> GLPTMNTPGSCQFLTSDDFQSPSAMPQYDVTPEMRIPGEVKNLMEIAEVDSVVPVQNVGEKVNSMEAYQIPVRSNEGSGTQVFGFPLQPGYSSVFSRTLLGEILNYYTHWSGSIKLTFMFCGSAMATGKFLLAYSPPGAGAPTKRVDAMLGTHVIWDVGLQSSCVLCIPWISQTHYRFVASDEYTAGGFITCWYQTNIVVPAD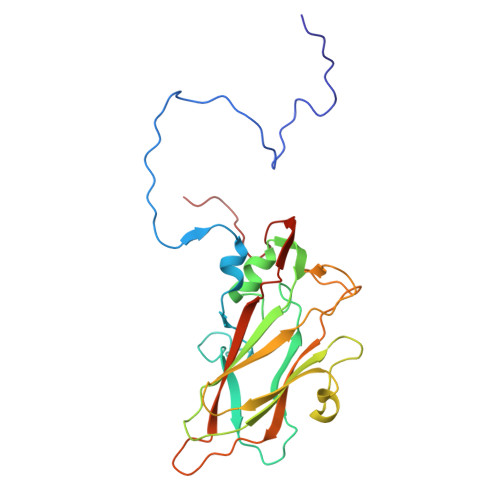AQSSCYIMCFVSACNDFSVRLLKDTPFISQQNFFQ1-{4-[(2-chloro-5-{1-[3-(4-cyclopropylpiperazin-1-yl)propyl]-5-(methylsulfonyl)-4,5,6,7-tetrahydro-1H-pyrazolo[4,3-c]pyridin-3-yl}phenyl)ethynyl]phenyl}-N-[(4-chlorophenyl)methyl]methanamine 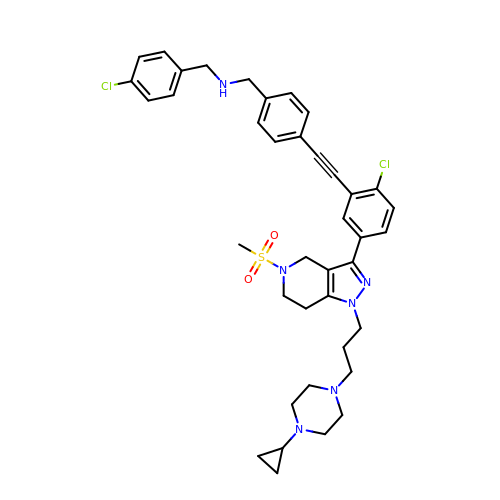| C39 H44 Cl2 N6 O2 S | HQHJSIFCCGLWGY-UHFFFAOYSA-N> QNGYENPT;> GSHMSRPPSREI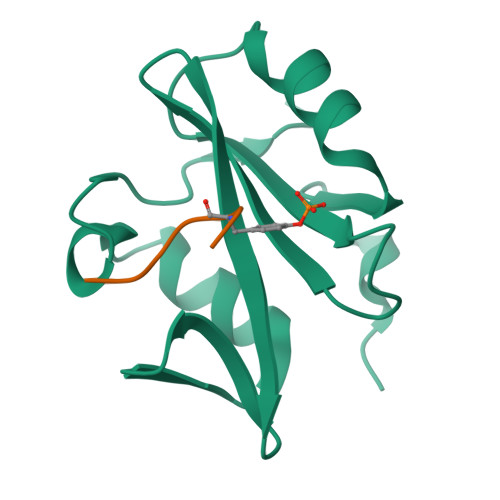DYTAYPWFAGNMERQQTDNLLKSHASGTYLIRERPAEAERFAISIKFNDEVKHIKVVEKDNWIHITEAKKFDSLLELVEYYQCHSLKESFKQLDTTLKYPYKSRE>SNANDLLP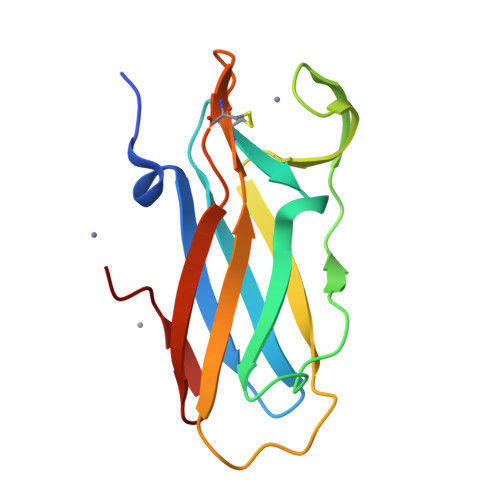PEKAFVPELAVADDGVNVRFRIADGYYMYQAKIVGKTDPADLLGQPSFSKGEEKEDEFFGRQTVYHHEAQVAFPYAKAVGEPYKLVLTYQGCAEVGVCYPPVDTEFDISGNGTYHPQT[6x]> SSSWRDHGI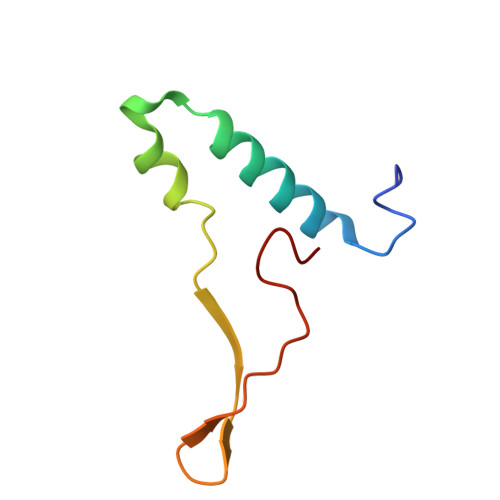SYLKYLNVCTETLHSTVKESRRAKYERWSKPCYTAQRPDGAGGQETIDKVPIHTKDY>MQRNTYNKVGLYILSLAMLFVFIIILTAKIPFCFTSDCSFIGLKKLVLTNIVPIVCFVFFLFSIYFYNRLKNITKYNGQDSVKITSCQSESYESLTFLATYIVPFMGFSFEDMQKNIAYLLLVVVIGIIFIKTDKYYANPTLALFGFKLYRVNILHPGSGETKNLIAISNDVLKVDDNVYYSFFDEFVFIARKKI[4x];>MTTQQLKEKISKIIDNFSGIRVVFTTTANELKLSRIEGSALNSIAEGFIDKIKEDIINNEDLTSPLLSNFDDRKNALFKFDYEQYPEEFNKITQAIAIPPNSQDYYNPLNKFTDVKGIIILISGDNKCLALYKNKTNLAVLRNSRKMFNLVPDPDGYLKQLPNEILRLDFNYDLFSIGEDFYIKNHKTLETQMKFHQVIEAQAVIALNSLRD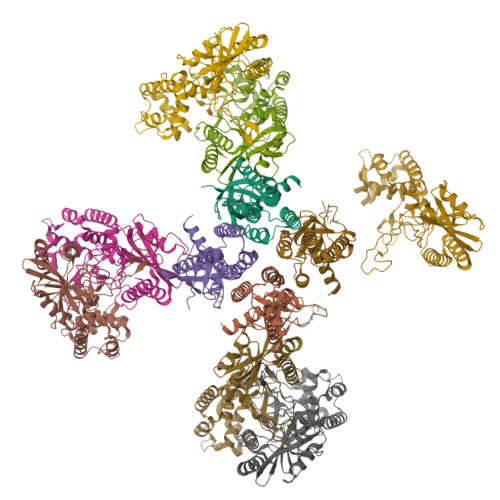SLLIEDISGLEKSSREISFARKLAKISKHSPVLGKIDTKTIIDYVSQHKYLSAILQINEAGDKLLIKTKTSQKHFIKLMSDDYLQSDLTKIIYMSIAKDRLDE[7x]>MSNVIQFYDIPGNATPDKAWSPNTWKTRYTLNFKGIPYKTIWVEYPDIASVCKEIGAEPTSIRPDGPYYTLPVIHDPSTGKTISDSAAIARYLDKTYPDTPVVIPPETDALHAAFNFAFSEAIVRALAP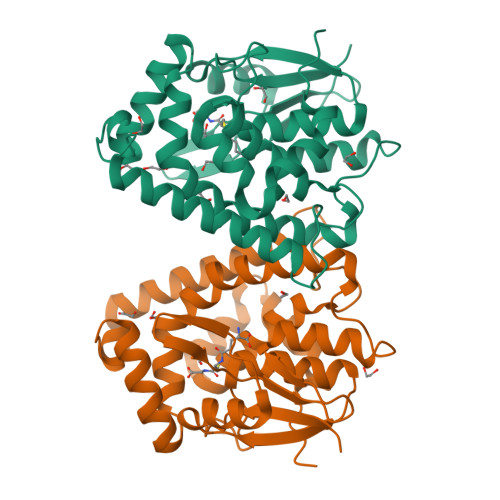IMLPATNAQLNPRSEEFFRRTREESAGGVKLEDWAPPGSEKRAKAWEKIRAGFGQIAKWLSADGNDKLLFLGDKVSYADITIVGWVIWVKRVLGPDSAEWKDFETWDDGKWAKQLALFEKYEVVPDA[2x]>GMRSNRVTQHPPLQLSLPVHLPDDETFTSYYPAAGNDELIGALKSAASGDGVQAIYLWGPVKSGRTHLIHAACARANELERRSFYIPLGIHASISTALLEGLEQFDLICIDDVDAVAGHPLWEEAIFDLYNRVAEQKRGSLIVSASASPMEAGFVLPDLVSRMHWGLTYQLQPMMDDEKLAALQRRAAMRGLQLPEDVGRFLLNRMARDLRTLFDVLDRLDKASMVHQR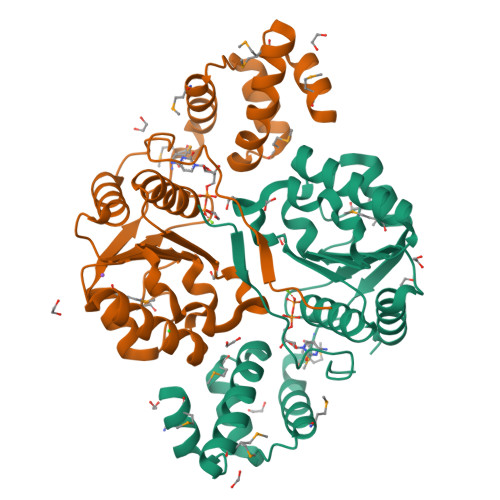KLTIPFVKEMLRL[2x]> SSAEQSFLFSREEADTLRLKVEELEGERSRLEEEKRMLEAQLERRALQGDYDQSRTKVLHMSLNPTSVARQRLREDHSQLQ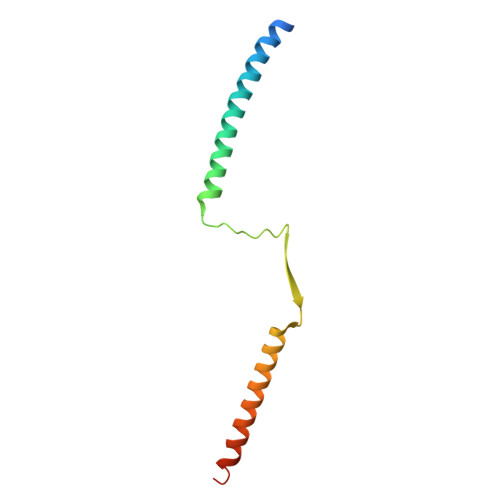AECERLRGLLRAMERGGTV>[4x]SGMATV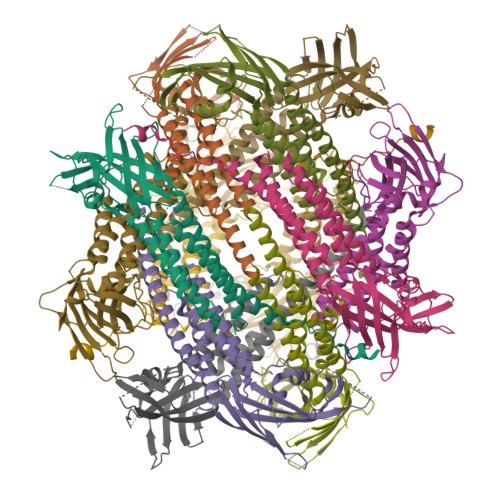MAATAAERAVLEEEFRWLLHDEVHAVLKQLQDILKEASLRFTLPGSGTEGPAKQENFILGSCGTDQVKGVLTLQGDALSQADVNLKMPRNNQLLHFAFREDKQWKLQQIQDARNHVSQAIYLLTSRDQSYQFKTGAEVLKLMDAVMLQLTRARNRLTTPATLTLPEIAASGLTRMFAPALPSDLLVNVYINLNKLCLTVYQLHALQPNSTKNFRPAGGAVLHSPGAMFEWGSQRLEVSHVHKVECVIPWLNDALVYFTVSLQLCQQLKDKISVFSSYWSYRPF> EVVSLTQAMISQYPAWSVGRSNLQALAGKTCGLAEDVLVELDPNAGMLAPVTAPLADALGAGLSEAFTPNGIPADVTADPVMERPGDRSFLNDDGLITGSEPGTEGGTTAAPGINGSRARLPYNLDPARTPVLGSWRAGVQVPAMLRSGWYRLPTNEQRDRAPLLVVTAAGRFDSREVRLQWATDEQAAAGHHGGSMEFADVGAAPAWRNLRAPLSAIPSTATQVRLVADDQDLAPQHWIALTPPRIPRVRTLQNVVGAADPVFLDWLVGLAFPCQRPFGHQYGVDETPKWRILPDRFGAEANSPVMDHNGGGPLGITELLMRATTVASYLKDDWFRDWGALQRLTPYYPDAQPADLNLGTVTRSGLWSPAPLRRGAPPPPPLGRDPNSSSVDKLAAALEH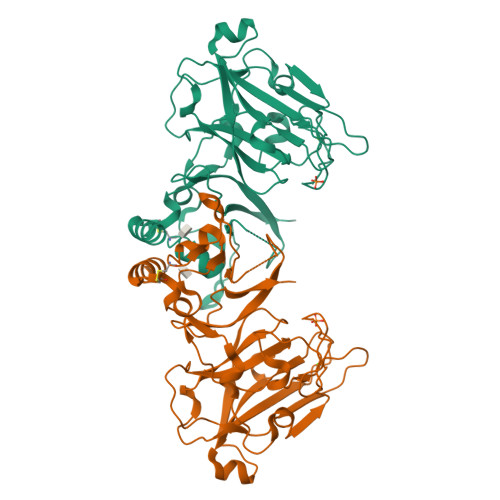HHHHH>MRVLVSNDDGVDAPGIKILADALRNAGHEVMVVAPDRDRSGASNSLTLDTPIRAKQIDMHTYSVAGTPTDC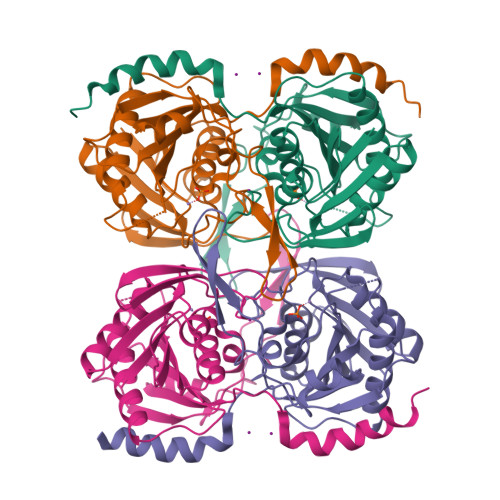VHLALTGLLNYDPDIVVSGINNTGNLGDDVIYSGTVSAAMEGRFLGLPAVAVSLVTLYREGQQAPQYETAAHAAINIVAQLKTDPLPADTILNVNVPDVTWQQMRGFKVTRLGNRHRSAPCLTQTDPRGHTIYWIGPAGPEQDAGPGTDFDAVRNTYISITPIHVDLTRYQALENVTRWTDRLTAHMDWPTLEHHHHHH[4x]> ELTPDQQTLLHFIMDSYNKQRMPQEITNKILKEEFSAEENFLILTEMATNHVQVLVEFTKKLPGFQTLDHEDQIALLKGSAVEAMFLRSAEIFNKKLPSGHSDLLEERIRNSG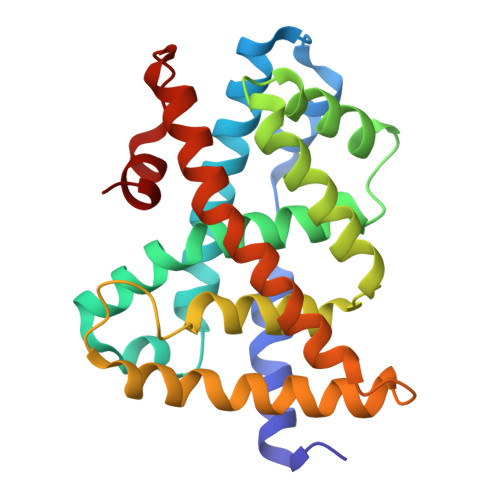ISDEYITPMFSFYKSIGELKMTQEEYALLTAIVILSPDRQYIKDREAVEKLQEPLLDVLQKLCKIHQPENPQHFAELLGRLTELRTFNHHHAEMLMSWRVNDHKFTPLLEEIWDV> KALYSKPGSKNGRWNPETHKFCKCGVRIQTSAYTCSKCRNRSGENNSFFNHKHSDITKSKISEKMKGKKPSNIKKISCDGVIFDCAADAARHFKISSGLV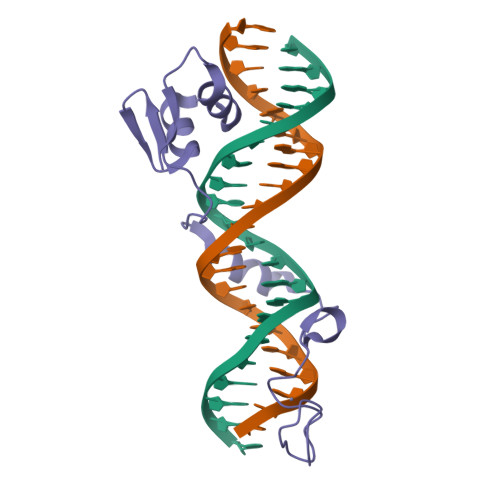TYRVKSDKWNWFYINA> MKKYTCTVCGYIYNPEDGDPDN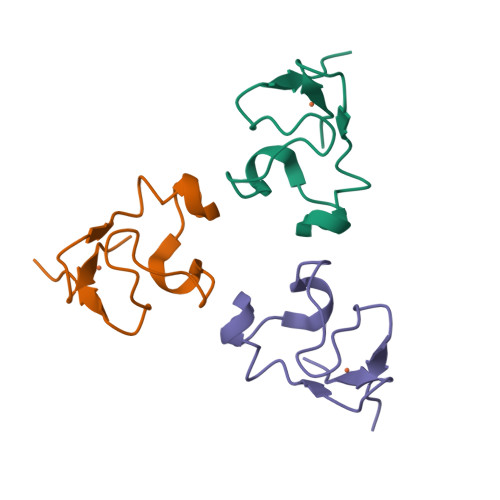GVNPGTDFKDIPDDWVCPLSGVGKDQFEEVEE>[4x]RVVCREASHAGSWYTASGPQLNAQLEGWLSQVQSTKRPARAIIAPHAGYTYCGSCAAHAYKQVDPSITRRIFILGPSHHVPLSRCALSSVDIYRTPLYDLRIDQKIYGELWKTGMFERMSLQTDEDEHSIEMHLPYTAKAMESHKDEFTIIPVLVGALSESKEQEFGKLFSKYLADPSNLFVVSSDFCHWGQRFRYSYYDESQGEIYRSIEHLDKMGMSIIEQLDPVSFSNYLKKYHNTICGRHPIGVLLNAITELQKNGMNMSFSFLNYAQSSQCRNWQDSSVSYAAGALTVH

Mediator of ERBB2-driven cell motility 1 (MEMO1) is an evolutionary conserved protein implicated in many biological processes; however, its primary molecular function remains unknown. MEMO1 is a highly conserved protein found in the cytosol of eukaryotic cells from yeast to humans. We conclude that MEMO1 is an iron-binding protein that modulates iron homeostasis in cancer cells. Our work reveals that the iron coordination mode in MEMO1 is very similar to that of iron-containing extradiol dioxygenases, which also display a similar structural fold.

To reveal the binding mode of each metal, we have crystallized MEMO1 in the presence of iron or copper under the conditions similar to those used previously for solving the structure of the metal-free protein. To prevent metal oxidation, MEMO1 crystallization with iron (II) or copper (I) was set up in an anaerobic chamber and the plates were incubated under argon, while the crystals were growing. In the MEMO1-Fe structure, iron density is clearly visible in the region of the previously predicted metal-binding site with an overall occupancy of 40–60%, as confirmed by the anomalous diffraction map. Iron is coordinated by H49, H81, and C244. Thus, iron coordination by two histidines and a cysteine in MEMO1 is an unusual variation on a common theme. A glutathione molecule was also found in the MEMO1-Fe structure, close to the iron-binding site, with the glutathione glycine carboxyl forming an electrostatic interaction with H192. This finding is consistent with Fe-GSH binding to MEMO1 observed by ITC. The protein fold of both metal-bound forms of MEMO1 is essentially identical to the metal-free structure, with RMSD for α-carbons of the superimposed structures being less than 0.17 Å. Inductively coupled plasma mass-spectrometry (ICP-MS) showed that, under these conditions, MEMO1 binds stoichiometric amounts of iron (approximately 1:1 molar ratio). The iron-binding site of MEMO1 is structurally very similar to that of iron-containing extradiol dioxygenases, with a notable difference of a cysteine residue (C244) located at the position occupied by a glutamate in those proteins.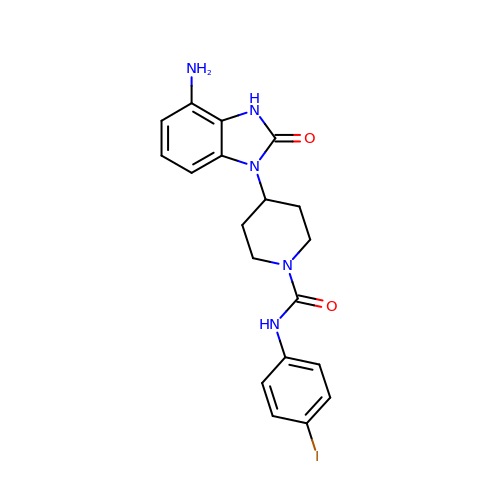4-(4-azanyl-2-oxidanylidene-3~{H}-benzimidazol-1-yl)-~{N}-(4-iodophenyl)piperidine-1-carboxamide | C19 H20 I N5 O2 | MCANHWLZFZFTAQ-UHFFFAOYSA-N7,8-DIAMINO-NONANOIC ACID | C9 H20 N2 O2 | 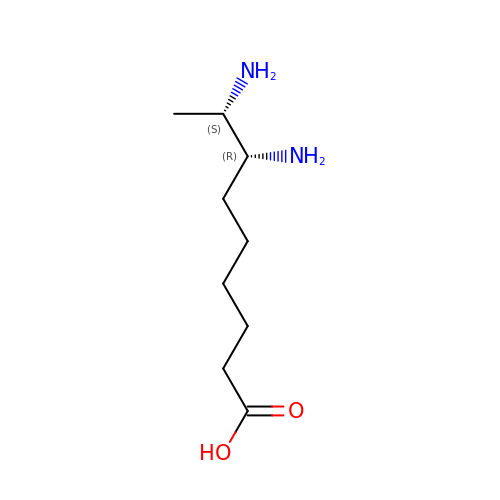KCEGBPIYGIWCDH-JGVFFNPUSA-N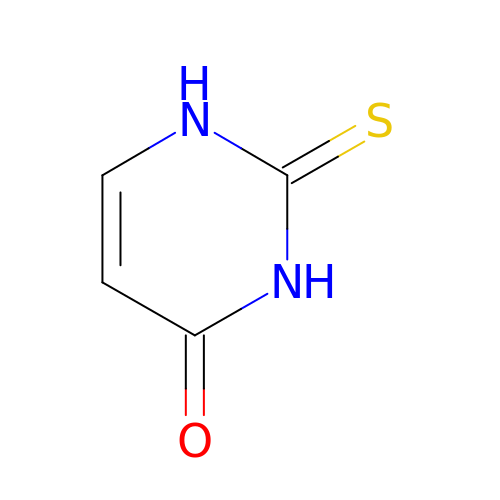2-thioxo-2,3-dihydropyrimidin-4(1H)-one | C4 H4 N2 O S | ZEMGGZBWXRYJHK-UHFFFAOYSA-N> MVARVQTAEEIRDEGNAAVKDQDYIKADELYTEALQLTTDEDKALRPVLYRNRAMARLKRDDFEGAQSDCTKALEFDGADVKALFRRSLAREQLGNVGPAFQDAKEALRLSPNDKGIVEVLQRLVKANNDKIKQTTSLANKVTDMEKLAFRGEAKDTEQKMTALNNLLVLCRESESGATGVWNQGALVPFVLNLINDASENEEVTVTAIRILDETIKNSVRCMKFLAMHDPDGPKSVRFVCRLMCKKSTKDFVDATGILVQRVFNAMAKMDRQKEMKPDPEVAEANKIWIIRVLLELQEMLQDPKVGAVQRETCIDLFLKNLMHMDGGIPRGWSWKFVEERGLLALLDVASQIPELCEYPVSAETRQHVAICLQRLEEDMVFDTKRTIFKEKVDMFFNALISRCTNDDEGHKYRIKLSCFLITMLQGPVDIGINLITNDQLTPIMLEMAASQDHLMQGIAAELIVATVSKHERAINMLKVGIPVLRALYDSEDPTVKVRALVGLCKIGAAGGDDISKATMKEEAVISLAKTCKKFLLETEKYSVDIRRYACEGLSYLSLDADVKEWIVDDSLLLKALVLLAKKAGALCVYTLATIYANLSNAFEKPKVDEEMVKLAQFAKHHVPETHPKDTEEYVEKRVRALVEEGAVPACVAVSKT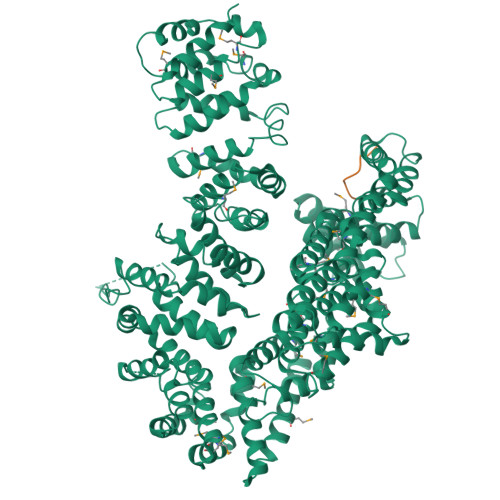ESKNALELIARSLLAFAEYEDLRGRIIAEGGTVLCLRLTKEASGEGKIKAGHAIAKLGAKADPMISFPGQRAYEVVKPLCDLLHPDVEGKANYDSLLTLTNLASVSDSIRGRILKEKAIPKIEEFWFMTDHEHLRAAAAELLLNLLFFEKFYEETVAPGTDRLKLWVLYSAEVEEERLSRASAAGFAILTEDENACARIMDEIKSWPEVFKDIAMHEDAETQRRGLMGIANIMHSSNKLCSEIVSSEVFRVLVAVTKLGTINQERAGSTEQAKRGLEAAEKFGLIKATDREIYERENQMSTIQE;> EDASRMEEVD> EV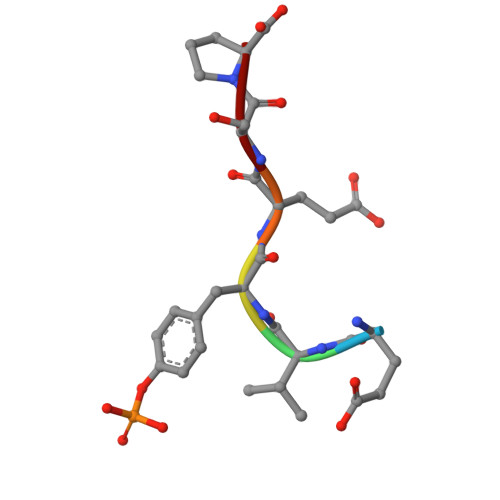YESP>GFKQDIATLRGDLRTYAQDIFLAFLNKYPDEKRNFKNYVGKSDQELKSMAKFGDHTEKVFNLMMEVADRATDCVPLASDASTLVQMKQHSGLTTGNFEKLFVALVEYMRAS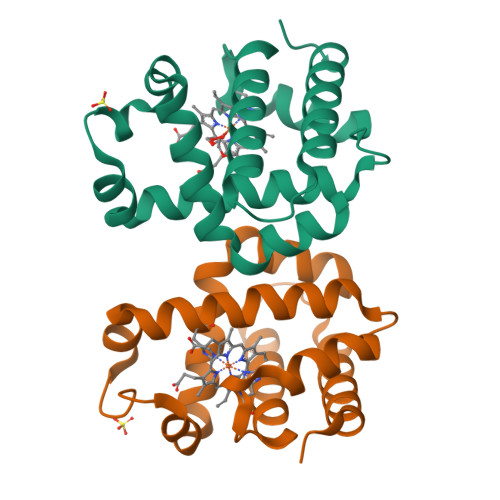GQSFDSQSWDRFGKNLVSALSSAGMK[2x]> GSMSTETLEIYRKALNFNVIARYDPKIKQLLFHTPHATVYKWGDDNWNKLEYQGVLAIYLRDVGDKEAILPEVSSYDDTITGQQSEANTPHVLTGHDIYNYGLIIMNRINPDNFSLAIAPNSVLNKRKLFAPNREEELEPMKVEVRDDLVMIKTLKKEVYGIWVHTPEDRQNIYE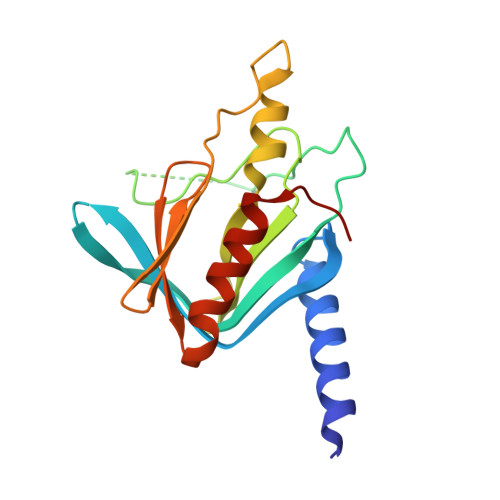LIKYLLENEPTDSFT> MKVAILSGSVYGTAEEVARHAQKLLSAAGLEASHLPRASLDELKAFAPEAFLVVTSTTGMGELPDNLQPLYYAIRD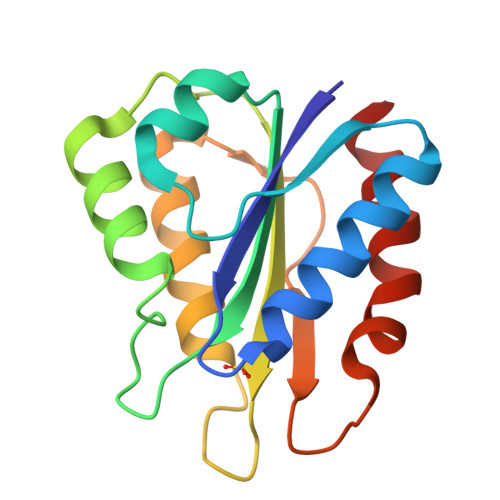QLPAWHGLPGGVIGLGDSSYGDTFAGGGEQVRELFGELGVREVLPMLRLDASETVTPETDAEPWLAEFAAALKG> FLVPPTVEQKTRPFTLPNLPLSSLSNSRAPLPISSMGISPDNVQSVQFQNGRCTLDGRLVGTTPVSLSHVAKIRGTSNGTVINLTELDGTPFHPFEGPAPIGFPDLGGCDWHINMTQFGHSSQTQYDVDTTPDTFVPHLGSIQANGIGSGNYVGVLSWISPPSHPSGSQVDLWKIPNYGSSITEATHLAPSVYPPGFGEVLVFFMSKMPGPGAYNLPCLLPQEYISHLASEQAPTVGEAALLHYVDPDTGRNLGEFKAYPDGFLTCVPNGA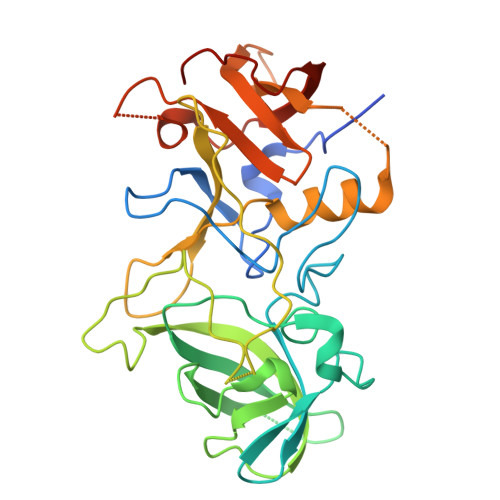SSGPQQLPINGVFVFVSWVSRFYQLKPVGTASSA>MQENQDGRYSLTYIYTGLSKHVEDVPAFQALGSLNDLQFFRYNSKDRKSQPMGL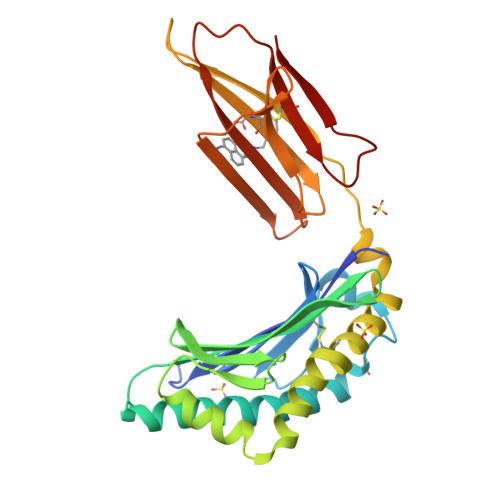WRQVEGMEDWKQDSQLQKAREDIFMETLKDIVEYYNDSNGSHVLQGRFGCEIENNRSSGAFWKYYYDGKDYIEFNKEIPAWVPFDPAAQITKQKWEAEPVYVQRAKAYLEEECPATLRKYLKYSKNILDRQDPPSVVVTSHQAPGEKKKLKCLAYDFYPGKIDVHWTRAGEVQEPELRGDVLHNGNGTYQSWVVVAVPPQDTAPYSCHVQHSSLAQPLVVPWEAS[6x]>[6x]MGNNLMQTDLSVWGMYQHADIVVKCVMIGL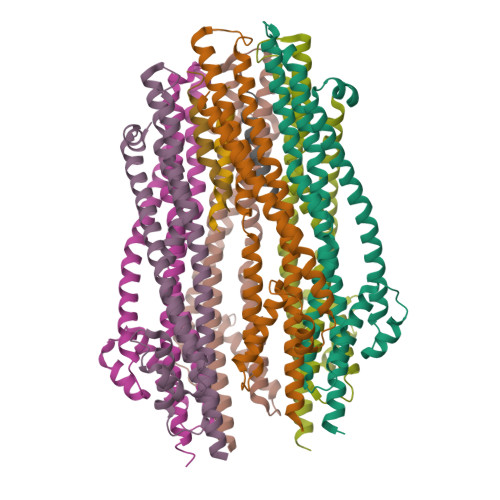ILASVVTWAIFFSKSVEFFNQKRRLKREQQLLAEARSLNQANDIAADFGSKSLSLHLLNEAQNELELSEGSDDNEGIKERTSFRLERRVAAVGRQMGRGNGYLATIGAISPFVGLFGTVWGIMNSFIGIAQTQTTNLAVVAPGIAEALLATAIGLVAAIPAVVIYNVFARQIGGFKAMLGDVAAQVLLLQSRDLDLEASAAAHPVRVAQKLRAG;>NVTPFIDVMLVLLIIFMVAAPL[3x]> XKVSALKEKVSALKEQFLM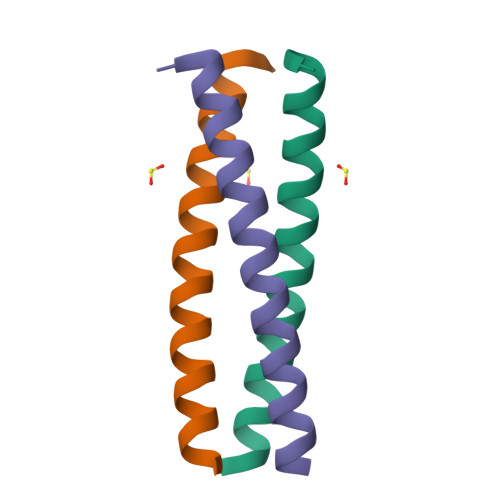LMFKVSALKEKVSALKE>MAIGEFMVSLPRMVYPQPKVLTPCRKDVLVVTPWLAPIVWEGTFNIDILNEQFRLQNTTIGLTVFAIKKYVAFLKLFLETAEKHFMVGHRVHYYVFTDQPAAVPRVTLGTGRQLSVLEVRAYKRWQDVSMRRMEMISDFCERRFLSEVDYLVCVDVDMEFRDHVGVEILTPLFGTLHPGFYGSSREAFTYERRPQSQAYIPKDEGDFYYGGAFFGGSVQEVQRLTRACHQAMMVDQA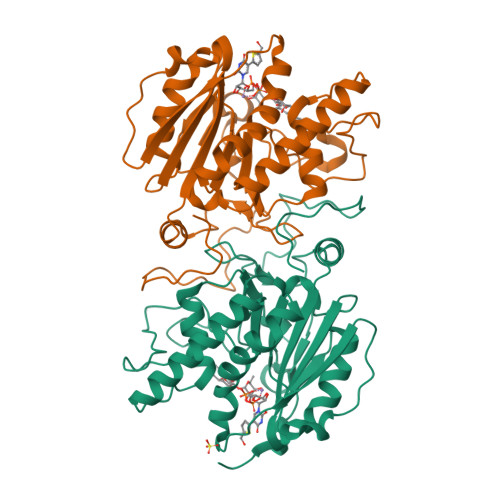NGIEAVWHDESHLNKYLLRHKPTKVLSPEYLWDQQLLGWPAVLRKLRFTAVPKNHQAVRNP[2x]> QYLLPEAKAQDSDKICVVINLDETLVHSSFKPVNNADFIIPVEIDGVVHQVYVLKRPHVDEFLQRMGELFECVLFTASLAKYADPVADLLDKWGAFRARLFRESCVF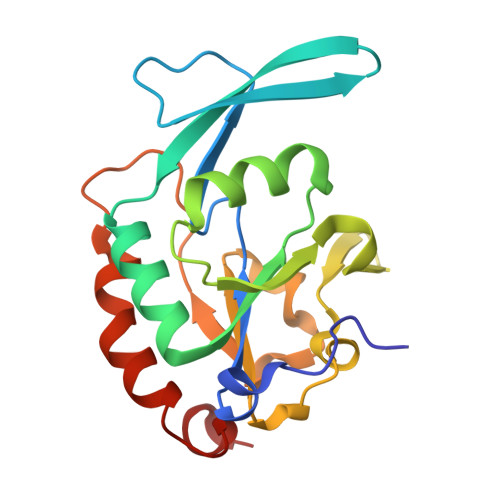HRGNYVKDLSRLGRDLRRVLILDNSPASYVFHPDNAVPVASWFDNMSDTELHDLLPFFEQLSRVDDVYSVLRQ>[2x]ATFDILNKCTYTVWAAASPGGGRRLDSGQSWTITVNPGTTNARIWGRTSCTFDANGRGKCETGDCNGLLECQGYGSPPNTLAEFALNQPNNLDYIDISLVDGFNIPMDFSGCRGIQCSVDINGQCPSELKAPGGCNNPCTVFKTNEYCCTDGPGSCGPTTYSKFFKDRCPDAYSYPQDDKTSLFTCPSGTNYKVTFCP

Despite these low concentrations, proteins have a great technological relevance in winemaking as some of them, the grape pathogenesis-related (PR) proteins, can aggregate to form a visible haze. Among the grape PR-proteins, the thaumatin-like proteins (TLPs) and chitinases can undergo changes in structural integrity, particularly under certain conditions such as when wines are exposed to elevated temperatures during storage or transportation. In this paper the crystal structure and some physico-chemical parameters relevant for the haze formation mechanism of three isoforms of TLPs isolated from grape juice were determined. Plant TLPs generally have three domains and a cleft located between domains I and II.

Despite sharing the same sequence, the two VVTL1 isoforms, I and H2 exhibited differences in their chromatographic behavior, a feature that allowed their separation and that also indicated that they possess some differences in physical properties. The physical differences between these two isoforms of the protein were also observed during crystallography. Although similar, distinctly different conditions were required to obtain crystals of the two proteins. The crystals of H2 were much smaller than those of I, hence diffraction data for these crystals were collected on the micro-crystallography beamline (MX2). Data were obtained up to 1.5∶Å, however there was a noticeable decrease in the quality of the last 60 images collected (out of 240), likely due to radiation damage, obliging us to cut the spot recognition to 2.5 σ, thus limiting the resolution to 1.65∶Å. The comparison of the two structures performed with the algorithm for protein structure alignment and comparison named TM-align tool indicated that the two proteins have a root mean square deviation (RMSD) of 0.78 Å, with a TM-score of 0.98, indicating that the proteins belong to the same fold (thaumatin), confirming results previously obtained with CATH. Differences were observed in loops between helixes α4 and α5 (loop A), between α5 and β13 (loop B) between β7 and β8 (loop C), and between β9 and β10 (loop D). These differences relate to alternate conformations of the loops between the two structures, rather than differences in the lengths of the loops. The solved crystal structures do not provide an explanation for their different chromatographic behavior, and this remains a topic for further study.> GPLGSPYTIELIQPEDGEAVIAMLKTFFFKDNPLNTFLDLGECKELEKYSLKPLPDNCSYKAVNKKGEIIGVFLNGLMRRPSPDDVPEKAADSCEHPKFKKILSLMD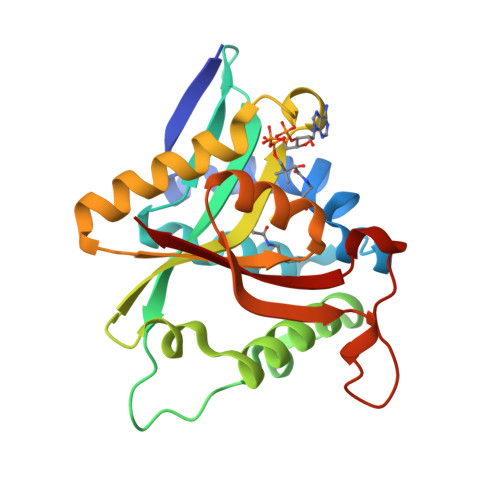HVEEQFNIFDVYPDEELILDGKILSVDTNYRGLGIAGRLTERAYEYMRENGINVYHVLCSSHYSARVMEKLGFHEVFRMQFADYKPQGEVVFKPAAPHVGIQVMAKEV> MEDLVSVGITHKEAEVEELEKARFESDEAVRDIVESFGLSGSVLLQTSNRVEVYASGARDRAEELGDLIHDDAWVKRGSEAVRHLFRVASGLESMMVGEQEILRQVKKAYDRAARLGTLDEALKIVFRRAINLGKRAREETRISEGAVSIGSAAVELAERELGSLHDKTV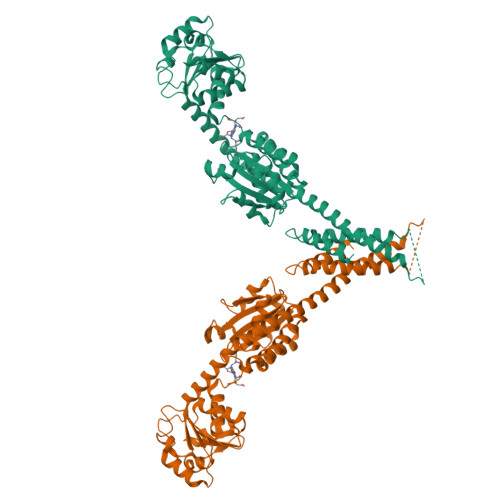LVVGAGEMGKTVAKSLVDRGVRAVLVANRTYERAVELARDLGGEAVRFDELVDHLARSDVVVSATAAPHPVIHVDDVREALRKRDRRSPILIIDIANPRDVEEGVENIEDVEVRTIDDLRVIARENLERRRKEIPKVEKLIEEELSTVEEELEKLKERRLVADVAKSLHEIKDRELERALRRLKTGDPENVLQDFAEAYTKRLINVLTSAIMELPDEYRRAASRALRRASELNG> GMPTDDIVQLLKGQEE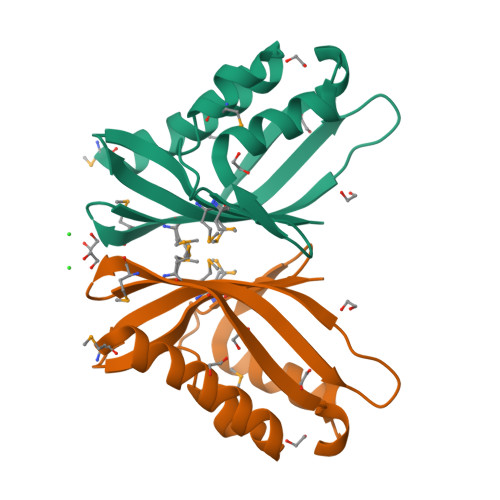AWNRGDLDAYMQGYWQNEQLMLISNGKFRNGWDETLAAYKKNYPDKESLGELKFTIKEIKMLSNYAAMVVGRWDLKRLKDTPTGVFTLLVEKIDDRWVITMDHSSD> NPVKREIHPDAVFYKEHKLRNDGLVITTNQGNIRLQFKSEAAIEVLYRADSKQLPSFALAQPESAIKAQLTETENHLQFSGGTLTARIQKRPFAISYYRDSELLLAEESGFQVNTDKINFRFYLSPGEKILGGGQRILGMDRRGQRFPLYNRAHYGYSDHSGQMYFGLPAIMSSKQYILVFDNSASGAMDIGKTESDILQLEAKSGRSAYILVAGNSYPSLIENFTQVTGRQPLPPRWALGSFASRFGYRSEAETRATVQKYKTEDFPLDTIVLDLYWFGKDIKGHMGNLDWDKENFPTPLDMMADFKQQGVKTVLITEPFVLTSSKRWDDAVKAKALAKDPQGQPKAFELYFGNGGIIDVFSKEGSRWFSSIYKDLSKQGVAGWWGNLGEPEMHPEDTQHAIGDADTVHNAYGHRWAEMLYQQQLDQFPELRPFIMMRAGFVGSQRYGMIPWTGDVSRTWGGLASQVELALQMSLLGFGYIHSDLGGFADGETLDKEMYIRWLQYGVFQPVYRPHGQDHIPSEPVFQDEETKAILRPLVKLRYRMLPYIYTAAYQNTLTGMPLMRPLFFSDEKNPALIDNKTSYFWGDSLLVTPITQAGVESVSIPAPKGVWFDFWKDTRYQTDGAPLTLPTDLHTIPVLVKAGAFMPYV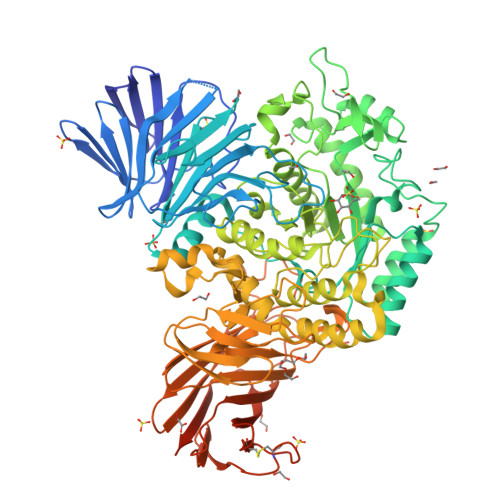PAVSTTEDYRSDSLEIHYYADASVPLAQGEIFEDDGKDPNSIKRNQFDLLTLQATHTDNQLHFQLARTGKGYRGMPERRATTLVIHNASDQYQHLDINGKTIAIAQADCASTPALACYDQERRQLQLVFTWGREALNLRLHKGGRADPAFLYKVVINSKLEGKPIPNPLLGLDSTRTGHHHHHH> MMFGRFTERAQKVLALAQEEALRLGHNNIGTEHILLGLVREGEGIAAKALQALGLGSEKIQKEVESLIGRGQEMSQTIHYTPRAKKVIELSMDEARKLGHSYVGTEHILLGLIREGEGVAARVLNNLGVSLNKARQQVLQLLGSNETGSSAAGTNSNANTPTLDSLARDLTAIAKEDSLDPVIGRSKEIQRVIEVLSRRTKNNPVLIGEPGVGKTAIAEGLAQQIINNEVPEILRDKRVMTLDMGTKYRGEFEDRLKKVMDEIRQAGNIILFIDAAIDASNILKPSLARGELQCIGATTLDEYRKYIEKDAALERRFQPIQVDQPSVDESIQILQGLRDRYEAHHRVSITDDAIEAAVKLSDRYISDRFLPDKAIDLIDEAGSKVRLRSFTTPPNLKELEQKLDEVRKEKDAAVQSQEFEKAASLRDTEQRLREQVEDTKKSWKEKQGQENSEVTVDDIAMVVS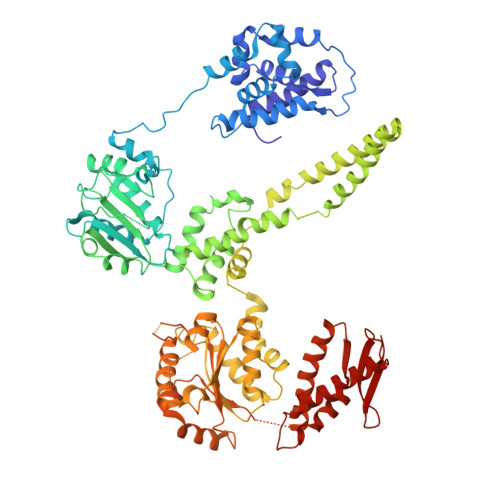SWTGVPVSKIAQTETDKLLNMENILHSRVIGQDEAVVAVAKAVRRARAGLKDPKRPIGSFIFLGPTGVGKTELARALAESIFGDEESMIRIDMSEYMEKHSTSGGQLTEKVRRKPYSVVLLDAIEKAHPDVFNILLQVLEDGRLTDSKGRTVDFRNTILIMTSNVGASEKDKVMGELKRAFRPEFINRIDEIIVFHSLEKKHLTEIVSLMSDQLTKRLKEQDLSIELTDAAKAKVAEEGVDLEYGARPLRRAIQKHVEDRLSEELLRGNIHKGQHIVLDVEDGEFVVKTTAKTN>MITVDITVNDEGKVTDVIMDGHADHGEYGHDIVCAGASAVLFGSVNAIIGLTSERPDINYDDNGGHFHIRSVDTNNDEAQLILQTMLVSLQTIE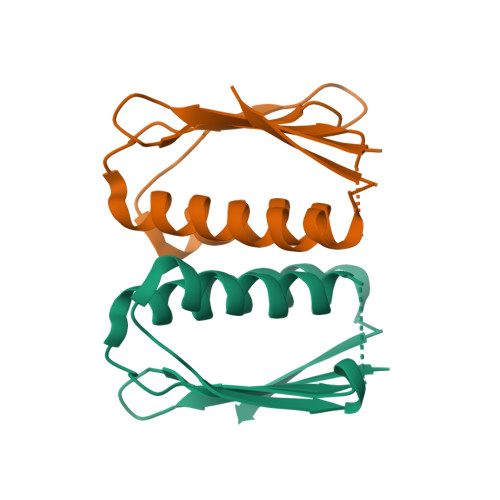EEYNENIRLNYK[2x]{2-[6-(2-ethyl-5-fluoro-4-hydroxyphenyl)-2H-indazol-3-yl]-3,4,6,7-tetrahydro-5H-imidazo[4,5-c]pyridin-5-yl}[5-(piperidin-1-yl)pyrazin-2-yl]methanone 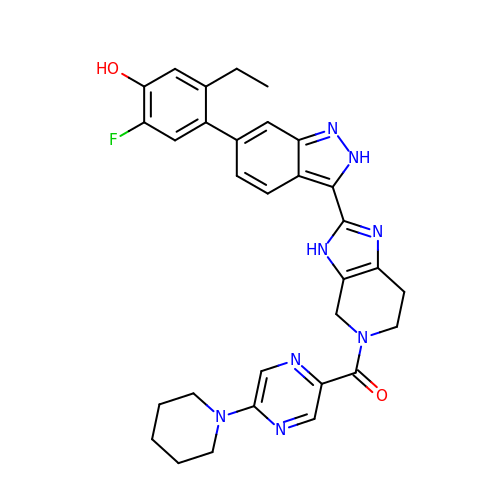| C31 H31 F N8 O2 | XDJGNPSZQSWJCV-UHFFFAOYSA-N>MQRGKVKWFNNEKGYGFIEVEGGSDVFVHFTAIQGEGFKTLEEGQEVSF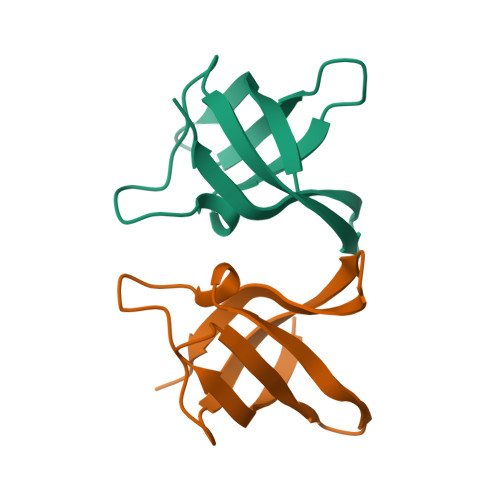EIVQGNRGPQAANVTKEA[2x]1-[4-[4-methyl-5-(3,4,5-trimethoxyphenyl)pyridin-3-yl]phenyl]piperazine | C25 H29 N3 O3 | 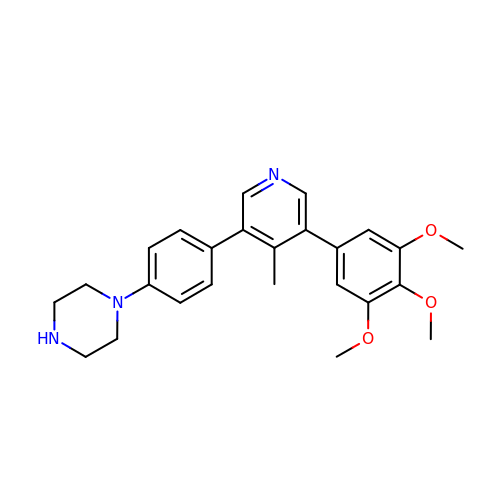RKBYYWVZFBATHQ-UHFFFAOYSA-N> SAPGEDEECGRVRDFVAKLANNTHQHVFDDLRGSVSLSWVGDSTGVILVLTTFHVPLVIMTFGQSKLYRSEDYGKNFKDITDLINNTFIRTEFGMAIGPENSGKVVLTAEVSGGSRGGRIFRSSDFAKNFVQTDLPFHPLTQMMYSPQNSDYLLALSTENGLWVSKNFGGKWEEIHKAVCLAKWGSDNTIFFTTYANGSCKADLGALELWRTSDLGKSFKTIGVKIYSFGLGGRFLFASVMADKDTTRRIHVSTDQGDTWSMAQLPSVGQEQFYSILAANDDMVFMHVDEPGDTGFGTIFTSDDRGIVYSKSLDRHLYTTTGGETDFTNVTSLRGVYITSVLSEDNSIQTMITFDQGGRWTHLRKPENSECDATAKNKNECSLHIHASYSISQKLNVPMAPLSEPNAVGIVIAHGSVGDAISVMVPDVYISDDGGYSWTKMLEGPHYYTI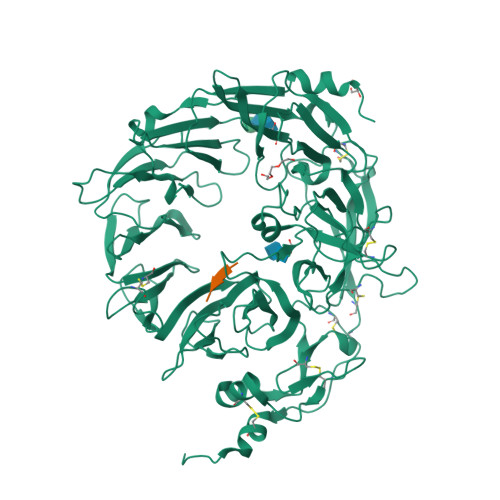LDSGGIIVAIEHSSRPINVIKFSTDEGQCWQTYTFTRDPIYFTGLASEPGARSMNISIWGFTESFLTSQWVSYTIDFKDILERNCEEKDYTIWLAHSTDPEDYEDGCILGYKEQFLRLRKSSMCQNGRDYVVTKQPSICLCSLEDFLCDFGYYRPENDSKCVEQPELKGHDLEFCLYGREEHLTTNGYRKIPGDKCQGGVNPVREVKDLKKKCTSNFLSPEKQNSKSNSHHHHHH;> QLYENKPRRPYIL>MNKLAVLYAEHIATLQKRTREIIERENLDGVVFHSGQAKRQFLDDMYYPFKVNPQFKAWLPVIDNPHCWIVANGTDKPKLIFYRPVDFWHKVPDEPNEYWADYFDIELLVKPDQVEKLLPYDKARFAYIGEYLEVAQALGFELMNPEPVMNFYHYHRAYKTQYELACMREANKIAVQGHKAARDAFFQGKSEFEIQQAYLLATQHSENDTPFGNIVALNENCAILHYTHFDRVAPATHRSFLIDAGANFNGYAADITRTYDFTGEGEFAELVATMKQHQIALCNQLAPGKLYGELHLDCHQRVAQTLSDFNIVNLSADEIVAKGITSTFFPHGLGHHIGLQVHDVGGFMADEQGAHQEPPEG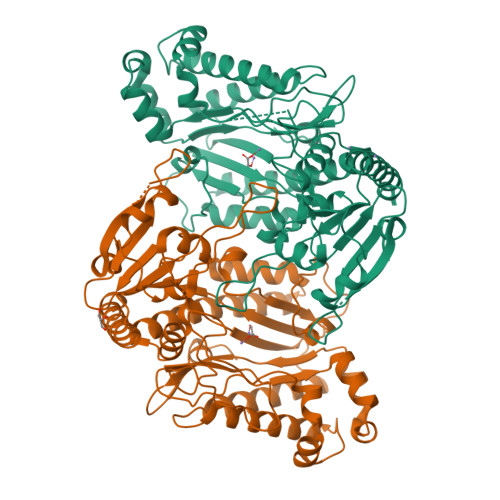HPFLRCTRKIEANQVFTIEPGLYFIDSLLGDLAATDNNQHINWDKVAELKPFGGIRIEDNIIVHEDSLENMTRELELD[2x]> MVNDLTPHFEDVQAHYDLSDDFFRLFLDPTQTYSCAHFEREDMTLEEAQIAKIDLALGKLGLQPGMTLLDIGCGWGATMRRAIAQYDVNVVGLTLSKNQAAHVQKSFDEMDTPRDRRVLLAGWEQFNEPVDRIVSIGAFEHFGHDRHADFFARAHKILPPDGVLLLHTITGLTRQQMVDHGLPLTLWLARFLKFIATEIFPGGQPPTIEMVEEQSAKTGFTLTRRQSLQPHYARTLDLWAEALQEHKSEAIAIQSEEVYERY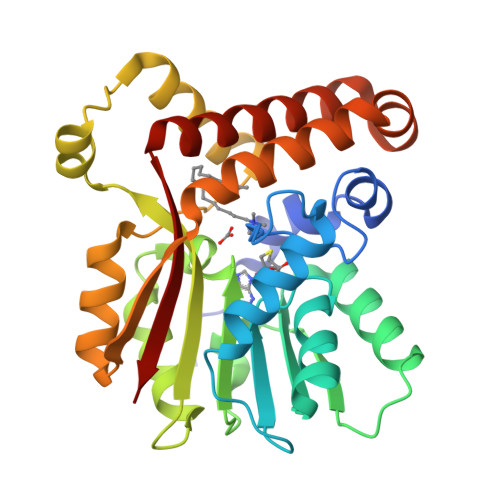MKYLTGCAKLFRVGYIDVNQFTLAK> MGNLFMLWAALGICCAAFSASAWSVNNFLITGPKAYLTYTTSVALGAQSGIEECKFQFAWERWNCPENALQLSTHNRLRSATRETSFIHAISSAGVMYIITKNCSMGDFENCGCDGSNNGKTGGHGWIWGGCSDNVEFGERISKLFVDSLEKGKDARALMNLHNNRAGRLAVRATMKRTCKCHGISGSCSIQTCWLQLAEFREMGDYLKAKYDQALKIEMDKRQLRAGNSAEGHWVPAEAFLPSAEAELIFLEESPDYCTCNSSLGIYGTEGRECLQNSHNTSRWERRSCGRLCTECGLQVEERKTEVISSCNCKFQWCCTVKCDQCRHVVSKYYC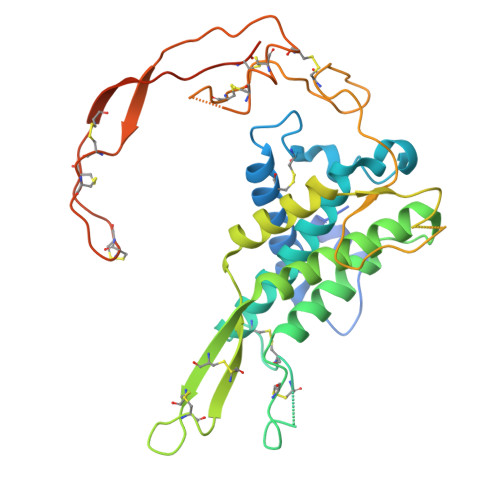ARSPGSAQSLGKGSAGGWSHPQFEK> MVTENPQRLTVLRLATNKGPLAQIWLASNMSNIPRGSVIQTHIAESAKEIAKASGCDDESGDNEYITLRTSGELLQGIVRVYSKQATFLLTDIKDTLTKISMLFKTSQKMTSTVNRLNTVTRVHQLMLEDAVTEREVLVTPGLEFLDDTTIPVGLMAQENSMERKVQGAAPWDTSLEVGRRFSPDEDFEHNNLSSMNLDFDIEEGPITSKSWEEGTRQSSRNFDTHENYIQDDDFPLDD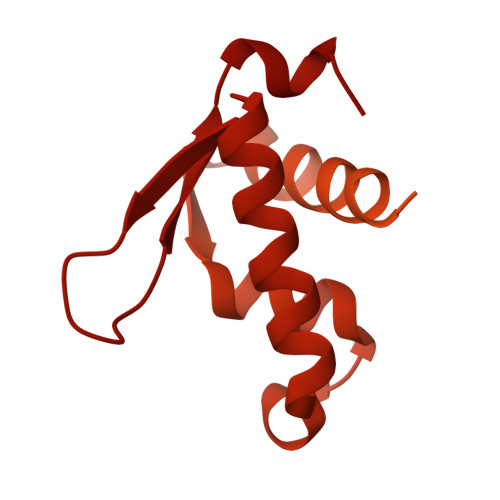AGTIGWDLGITEKNDQNNDDDDNSVEQGRRLGESIMSEEPTDFGFDLDIEKEAPAGNIDTITDAMTESQPKQTGTRRNSKLLNTKSIQIDEETENSESIASSNTYKEERSNNLLTPQPTNFTTKRLWSEITESMSYLPDPILKNFLSYESLKKRKIHNGREGSIEEPELNVSLNLTDDVISNAGTNDNSFNELTDNMSDFVPIDAGLNEAPFPEENIIDAKTRNEQTTIQTEKVRPTPGEVASKAIVQMAKILRKELSEEKEVIFTDVLKSQANTEPENITKREASRGFFDILSLATEGCIGLSQTEAFGNIKIDAKPALFERFINA>[2x]MKAIPPKIWFETQLKGSGLDKKFQIDELIETQSSVRVFANKKYLPDTETINEALTKVTAVNVSGDKSGYFQNGLPFPNEAGYFEKIPVGHPELLSPIERLTGSKKIVSSHSLVTASGGYPLTNPLLPYRKPIRVSIFSLAGPSFENNYLHYRLFLLDSVQKIIDSPLFSHLHDGLPIQFDEAKKELGEYDTNKLMARIRLGFPYLARFSSGGFYPSFSK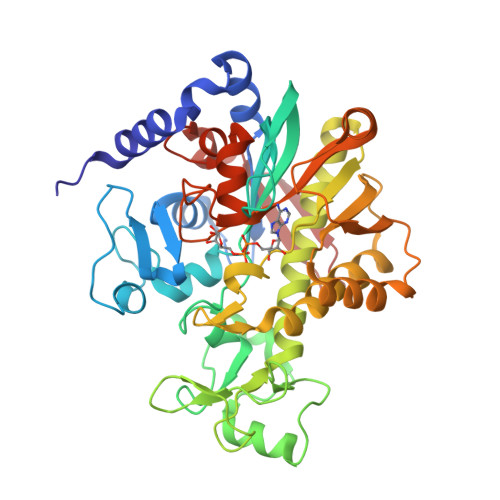SNAIIFLSEAYFRYQLEDVSLLLASVNQTGKETGKAALLKATAVGMGFFAKIDCGYDIQHIIFPYYLRAYKKLLSEHKFPWIAKIEFPIFNEIQQEQFDSIFEDYDGPTKVYRSTRDVLEFREEEIEKYLPAAINPSDAFALTGNEWGYGSVESMIGNNSSIRFDQVHHMNPLILDPSHHVEAQINKDHGVELTVN> 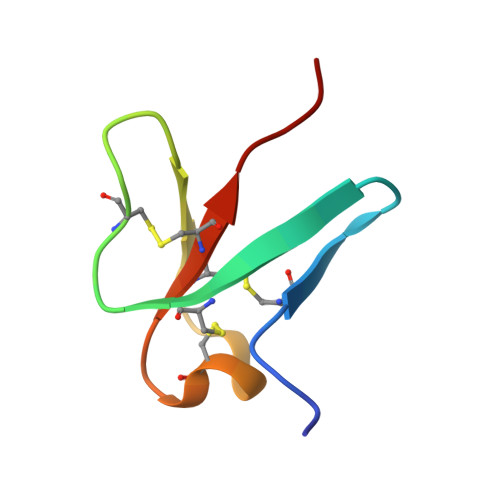ESGNSCYIYHGVSGICKASCAEDEKAMAGMGVCEGHLCCYKTPW>MIRLYPEQLRAQLNEGLRAAYLLLGNDPLLLQESQDAVRQVAAAQGFEEHHTFSIDPNTDWNAIFSLCQAMSLFASRQTLLLLL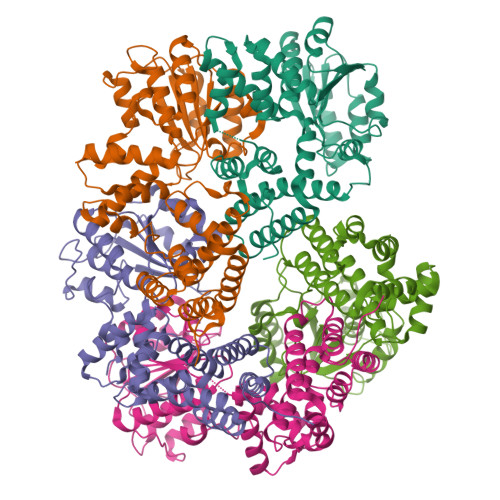PENGPNAAINEQLLTLTGLLHDDLLLIVRGNKLSKAQENAAWFTALANRSVQVTCQTPEQAQLPRWVAARAKQLNLELDDAANQVLCYCYEGNLLALAQALERLSLLWPDGKLTLPRVEQAVNDAAHFTPFHWVDALLMGKSKRALHILQQLRLEGSEPVILLRTLQRELLLLVNLKRQSAHTPLRALFDKHRVWQNRRGMMGEALNRLSQTQLRQAVQLLTRTELTLKQDYGQSVWAELEGLSLLLCHKPLADVFIDG[3x];>[9x]GPHMSYQVLARKWRPQTFADVVGQEHVLTALANGLSLGRIHHAYLFSGTRGVGKTSIARLLAKGLNCETGITATPCGVCDNCREIEQGRFVDLIEIDAASRTKVEDTRDLLDNVQYAPARGRFKVYLIDEVHMLSRHSFNALLKTLEEPPEHVKFLLATTDPQKLPVTILSRCLQFHLKALDVEQIRHQLEHILNEEHIAHEPRALQLLARAAEGSLRDALSLTDQAIASGDGQVSTQAVSAMLGTLDDDQALSLVEAMVEANGERVMALINEAAARGIEWEALLVEMLGLLHRIAMVQLSPAALGNDMAAIELRMRELARTIPPTDIQLYYQTLLIGRKELPYAPDRRMGVEMTLLRALAFHPRMPLPEPEVPRQ;>[3x]MRWYPWLRPDFEKLVASYQAGRGHHALLIQALPGMGDDALIYALSRYLLCQQPQGHKSCGHCRGCQLMQAGTHPDYYTLAPEKGKNTLGVDAVREVTEKLNEHARLGGAKVVWVTDAALLTDAAANALLKTLEEPPAETWFFLATREPERLLATLRSRCRLHYLAPPPEQYAVTWLSREVTMSQDALLAALRLSAGSPGAALALFQGDNWQARETLCQALAYSVPSGDWYSLLAALNHEQAPARLHWLATLLMDALKRHHGAAQVTNVDVPGLVAELANHLSPSRLQAILGDVCHIREQLMSVTGINRELLITDLLLRIEHYLQPGVVLPVPHL> SQSADERIGTFLNQADWFGLEKNYPILKDSMQADFLKLMSEALIGYYFNRPDEALQSIHKLLVNHQAEIGGQNALNMAILACQIDGLKGNYATAAQNSRSIMEQLKQQSAEQGMYKSLEGICYFYDQLKNIPAPGITCPQEDIIIPVDIEKVKLPTSIEPKGWRGTTILIPVTINGKTYQFIFDTGAGTSYMSQRMAKETGVRILSDSLVINSNLPGAMTGNFGTLENMQIGSITFHNSLITI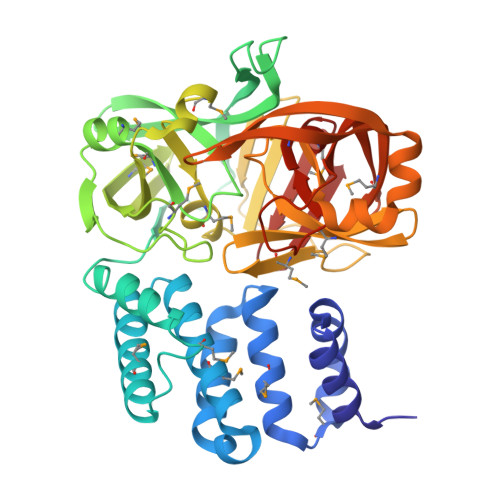APPNEFDSIMIVDAVLGMDFIGLFDEVRIYPKDKKIVFPKSSTPLPSYGRNLMKVDRALKLKAQANGETLMLHFDTGNSTAGLFYQYYEKHKAEFESIGKKEKITGGGFNHVVTKDILRLPSFDMEIGDATAHLKNLAVDITPNGIPAEDDGNIGMDMINQFDCVTINLKDMFLKLE>[2x]MKGSEEAYLVSDKATKMYSLTKDSEKNHPSKPPLQDEENPQSKYHCHNNNKKAYDARQREQTFAKKKLCIASLICFVFISAEIVGGYIAGSLAVVTDAAHLLVDLSSFFISLCSLWLSSKSSTTRLTFGWHRAEILGALMSVITIWLVTGVLVYLACERLIRPDYTIDGTVMLITSACALGA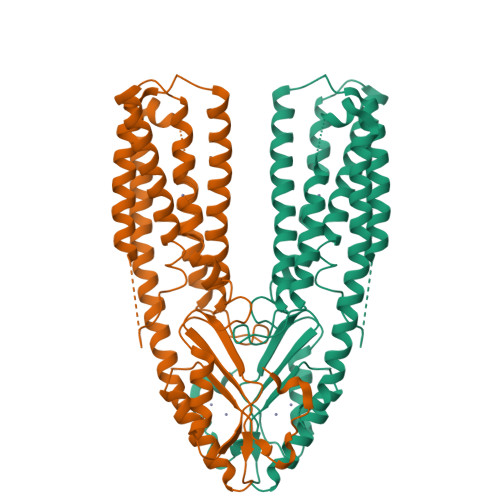NLVLALILHQSGHGHSHAGGKHEHMASEYKPQTNASIRAAFIHVIGDLFQSISVLISALIIYFKPEYKMADPICTFIFSIFVLITTVTVLRDLLTVLMEGTPRGIHYSDVKQSILAVDGVKSVHSLHLWALTMNQVILSAHIATDIVGESKRILKDVTQNVFARFPFHSVTIQVEPIEDQSPECMFCYEPTQ> IVGGTSASAGDFPFIVSISRNGGPWCGGSLLNANTVLTAAHCVSGYAQSGFQIRAGSLSRTSGGITSSLSSVRVHPSYSGNNNDLAILKLSTSIPSGGNIGYARLAASGSDPVAGSSATVAGWGATSEGGSSTPVNLLKVTVPIVSRATCRAQYGTSAIT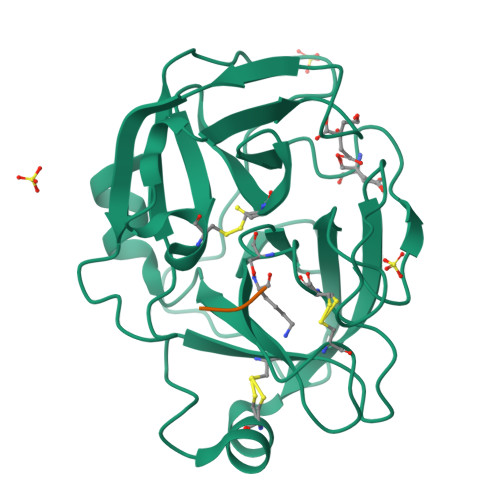NQMFCAGVSSGGKDSCQGDSGGPIVDSSNTLIGAVSWGNGCARPNYSGVYASVGALRSFIDTYA;> GGR> AKTEQQIADIVNRTITPLMQEQAIPGMAVAIIYEGKPYYFTWGKADI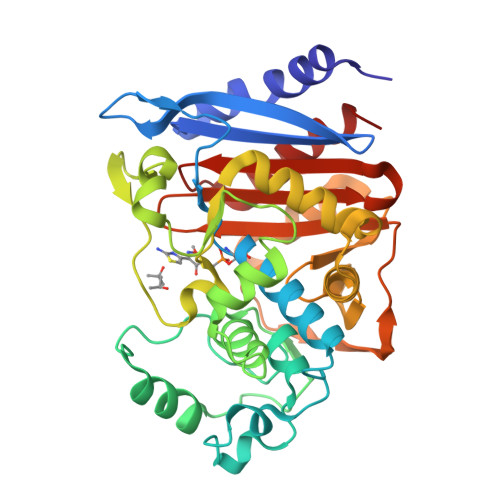ANNHPVTQQTLFELGSVSKTFNGVLGGDAIARGEIKLSDPVTKYWPELTGKQWRGISLLHLATYTAGGLPLQIPDDITDKAALLRFYQNWQPQWTPGAKRLYANSSIGLFGALAVKPSGMSYEEAMTRRVLQPLKLAHTWITVPQSEQKNYAWGYREGKPVHVSPGQLDAEAYGVKSSVIDMARWVQANMDASHVQEKTLQQGIELAQSRYWRIGDMYQGLGWEMLNWPLKADSIINGSDSKVALAALPAVEVNPPVPAVKASWVHKTGSTGGFGSYVAFVPEKNLGIVMLANKSYPNPVRVEAAWRILEKLQ>MFSRPGLPVEYLQVPSASMGRDIKVQFQGGGPHAVYLLDGLRAQDDYNGWDINTPAFEEYYQSGLSVIMPVGGQSSFYTDWYQPSQSNGQNYTYKWETFLTREMPAWLQANKGVSPTGNAAVGLSMSGGSALILAAYYPQQFPYAASLSGFLNPSEGWWPTLIGLAM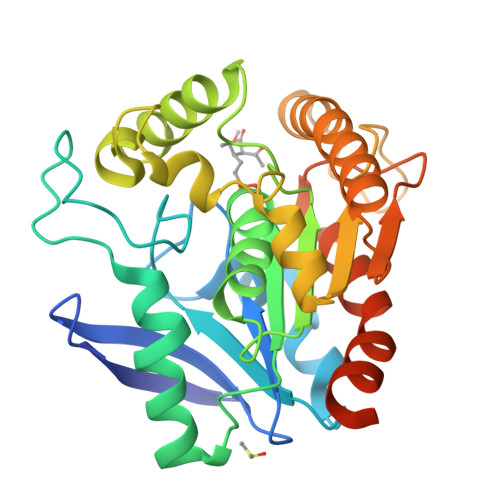NDSGGYNANSMWGPSSDPAWKRNDPMVQIPRLVANNTRIWVYCGNGTPSDLGGDNIPAKFLEGLTLRTNQTFRDTYAADGGRNGVFNFPPNGTHSWPYWNEQLVAMKADIQHVLNGATPPAAPAAPAALEHHHHHH[2x]>GAMVAANGSQRPIIAFMSDLGTTDDSVAQCKGLMHSICPGVTVVDVCHSMTPWDVEEGARYIVDLPRFFPEGTVFATTTYPATGTTTRSVAVRIRQAAKGGARGQWAGSGDGFERADGSYIYIAPNNGLLTTVLEEHGYIEAYEVTSTKVIPANPEPTFYSREMVAIPSAHLAAGFPLAEVGRRLDDSEIVRFHRPAVEISGEALSGVVTAIDHPFGNIWTNIHRTDLEKAGIGQGKHLKIILDDVLPFEAPLTPTFADAGAIGNIAFYLNSRGYLSLARNAASLAYPYNLKAGLKVRVEAR[2x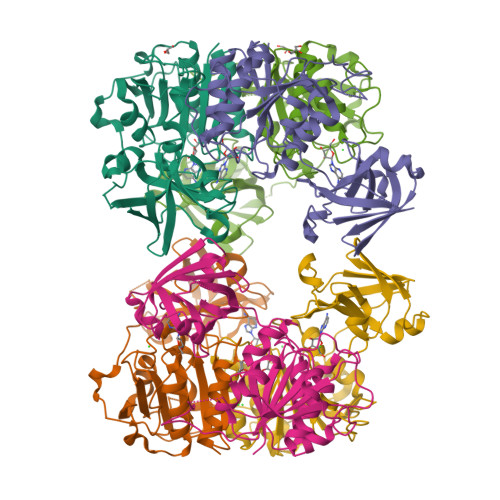]4-carboxy-1,1-dimethylpiperidin-1-ium | 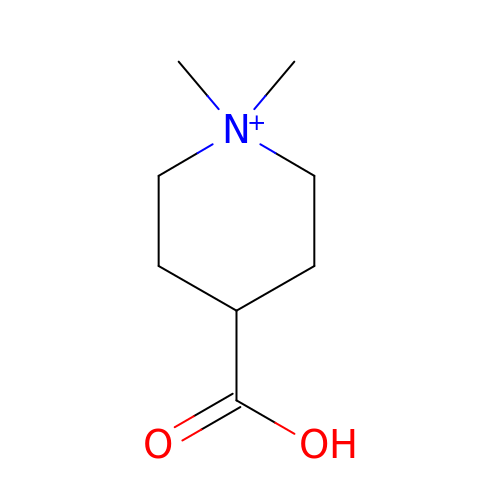C8 H16 N O2 | ZUZDUOOCVXTRAU-UHFFFAOYSA-O> VDYNAPLNPKSELFLDDWHIPKFNRFISFTLDVLIDKYKDIFKDFIKLPSRKFHPQYYYKIQQPMSINEIKSRDYEYEDGPSNFLLDVELLTKNCQAYNEYDSLIVKNSMQVVMLIEFEVLKAKNLKRNYLINSEVKAKLLHYLNKLVDATEKKINQALLGASSPKNLDDKVKLSEPFMELVDKDELPEYYEIVHSPMALSIVKQNLE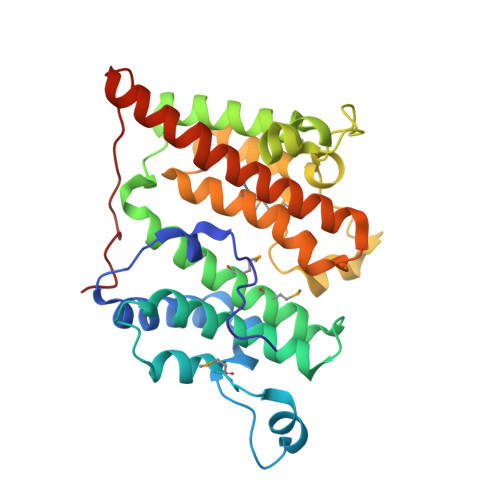IGQYSKIYDFIIDMLLVFQNAHIFNDPSALIYKDATTLTNYFNYLIQKEFFPELQDLNERGEINLEFDKFEFENYLA> MHADGAAAETAAPGQSAIENFQPVTAEDLAGGNAANWPILRGNYQGWGYTQLDQINKDNVGQLQLAWARTMEPGSNEGSAIAYNGVVFLGNANDVVQAIDGKTGNLIWEYRRKLPPASKFINSLGAAKRSIALFGDKVYFVSWDNFVVALDAKTGKLAWETNRGQGVEEGVSNSSGPIVVDGVVIAGSTCQYSGFGCYVTGTDAESGEELWRNTFIPRPGEEGDDTWGGAPYENRWMTGAWGQITYDPELDLVYYGSTGAGPASEVQRGTEGGTLAGTNTRFAVKPKTGEVVWKHQTLPRDNWDSECTFEMMVVSTTVNPDAGADGMMSVGANVPRGETRKVLTGVPCKTGVAWQFDAETGDYFWSKATVEQNSIASIDDKGLVTVNEDMILKEPGKDYNYCPTFLGGRDWPSAGYLPKSNLYVIPLSNACYDLKARTTEATPADVYNTDSTVKLAPGKTNMGRVDAIDVATGATKWSFETEAALYDPVMTTAGDLVFVGSTDRMFRALDAETGKEVWSTRLPGAISGYTTSYSIDGRQYVAVVAGGSLGTGFFKAAVPGVDAVQGGNGI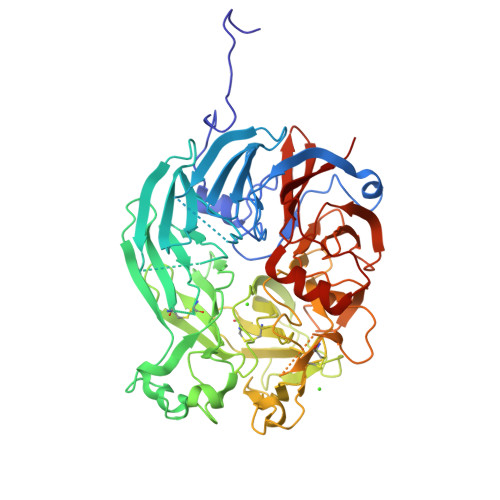YVFALPEAK> AAAAA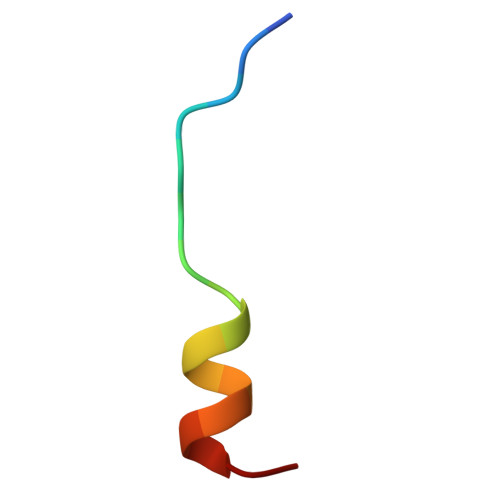AAAAAAAAAAAA>[4x]MNGERIIAFQGRPGAYSDLACRQARPGWTTLPCQTFAQTIAAVHDGRAELAMLACENSLAGRVPDIHALLPEAGLFIVGEHFQRVEHCLLGIPGSTLADARR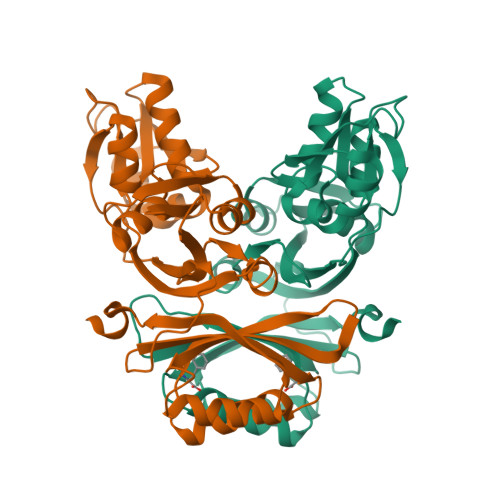IHTHPVAMAQVRGIITELGLDPVVEFDTAGAAEMVREWGRKEDVAVASALAAELNGLEILRRNVEDATHNTTRFYIASRRPATLPPPGPGFMTTLLFRVNNQPGALYKALGGLATAGVNMTRLESYMLEGSFSATQFLMDVEGHPEAPPLARALDELSFFSEQQEILGVYPASPFRRKP(~{E})-3-[4-oxidanyl-3-(3-propan-2-ylphenyl)phenyl]prop-2-enoic acid | C18 H18 O3 | 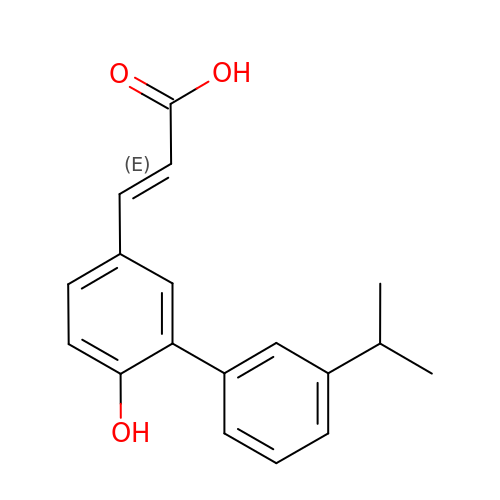CIHKFLQGYXDCJN-VQHVLOKHSA-N>[2x]GAFGGLPSLKSSFVLSEDTIPGTNETVKTLLPYGSVINYYGYVKPGQAPDGLVDGNKKAYYLYVWIPAVIAEMGVRMISPTGEIGEPGDGDLVSDAFKAATPEEKSMPHWFDTWIRVERMSAIMPDQIAKAAKAKPVQKLDDDDDGDDTYKEERHNKYNSLTRIKIPNPPKSFDDLKNIDTKKLLVRGLYRISFTTYKPGEVKGSFVASVGLLFPPG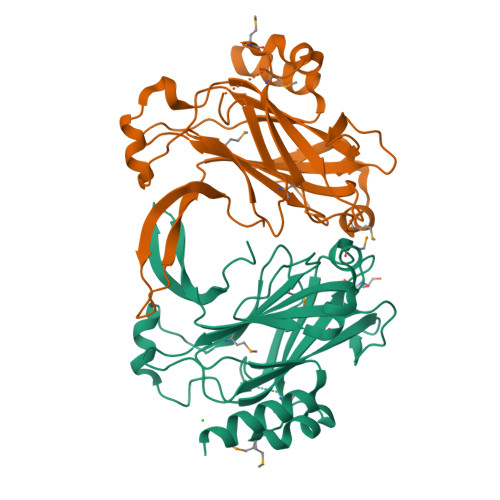IPGVSPLIHSNPEELQKQAIAAEESLKKAASDATK>[2x]GSQIHVDTMKVINDPIHGHIELHPLLVRIINTPQFQRLRYIKQLGGGYYVFPGASHNRFEHSLGVGYLAGCLVHALGEKQPELQISERDVLCVQIAGLCHDLGHGPFSHMFDGRFIPLARPEVKWTHEQGSVMMFEHLINSNGIKPVMEQYGLIPEEDICFIKEQIVGPLESPVEDSLWPYKGRPENKSFLYEIVSNKRNGIDVDKWDYFARDCHHLGIQNNFDYKRFIKFARVCEVDNELRICARDKEVGNLYDMFHTRNSLHRRAYQHKVGNIIDTMITDAFLKADDYIEITGAGGKKYRISTAIDDMEAYTKLTDNIFLEILYSTDPKLKDAREILKQIEYRNLFKYVGETQPTGQIKIKREDYESLPKEVASAK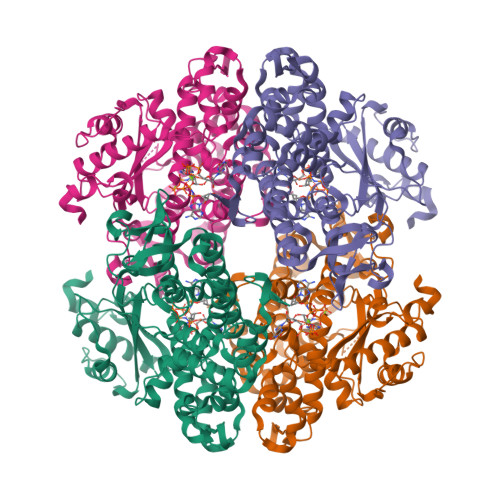PKVLLDVKLKAEDFIVDVINMDYGMQEKNPIDHVSFYCKTAPNRAIRITKNQVSQLLPEKFAEQLIRVYCKKVDRKSLYAARQYFVQWCADRNFTKPQDGDVIAPLITPQKKEWNDSTSVQNPTRLREASKSRVQLFKDDPM>[2x]SGLKKFFPYSTNVLKGAAADIALPSLAGKTVFFYFSASWCP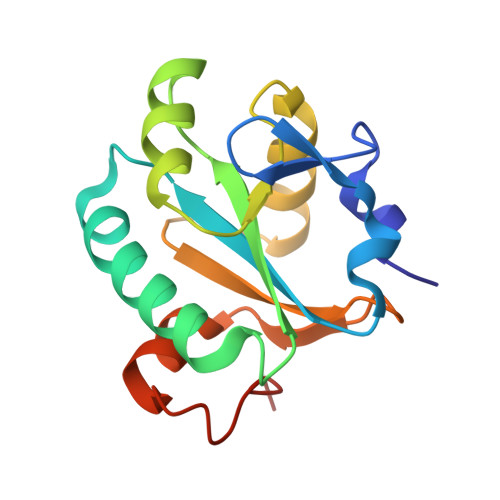PCRAFTPQLIDFYKAHAEKKNFEVMLISWDESAEDFKDYYAKMPWLALPFEDRKGMEFLTTGFDVKSIPTLVGVEADSGNIITTQARTMVVKDPEAKDFPWPNVEAKK Here, we describe a phage tailspike protein, named K2-2, that specifically depolymerizes the K2 capsular polysaccharide (CPS) of K. pneumoniae into tetrasaccharide repeating units. During the initial stage of infection, the tailspike proteins (TSPs) of bacteriophage recognize specific polysaccharides on the surface of the host cell and attach to them for adsorption. TSPs, also known as polysaccharide depolymerases, have the function of binding and digesting CPS. TSPs typically consist of three domains: an N-terminal particle-binding domain that connects to the tail structure or baseplate of the phage, a receptor-binding domain that extends from the homotrimeric structure and is responsible for host recognition and catalytic activity, and a C-terminal domain that plays a vital role in trimer formation, receptor binding, and intra-molecular chaperone functions.

Before the trimeric wild-type structures were determined using the N-terminally His-tagged protein, the first crystals of K2-2 were, indeed, obtained by using a C-terminally His-tagged protein (termed K2-2C-His). The structure was solved at 2.17 Å resolution by the MAD phasing method under the space group of P63. Unexpectedly, the solved structure revealed four protomers of the enzyme in an asymmetric unit, which formed a tetramer without the presence of a trimer. Specifically, two subunits are assembled into a dimer of a parallel left-handed helix, and two such dimers combine to form a right-handed superhelix. The two dimers superimpose well with each other, and also with any two adjacent subunits in the trimeric wild-type structure, presumably sharing a common interface. Regardless of the different overall organization, individual subunit in the tetrameric structure of K2-2C-His exhibited a conformation nearly identical to that in the trimeric form. The intersubunit carbohydrate-binding groove could be overlaid well with that of the trimeric structure (Cα rmsd = 0.29 Å), including the residues involved in binding the sugar (Fig. 5B through C). Notably, as determined by top agar assay, this tetrameric form of K2-2C-His possessed a significant capsule degradation activity towards the K2 K. pneumoniae. Conceivably, although the electron density corresponding to the C-terminal His-tag was not visible in all subunits, the protruding His-tag might give rise to steric hindrance that interfered with the assembly of the enzyme into a trimer. Finally, the structural and functional characterization of the tetrameric form of K2-2 here demonstrates, for the first time in the field of TPSs, that a functional intersubunit catalytic center could be formed without the need for trimerization.

>MALVDLVRAGGYSVEYPQFSSMAKLKAFPHSEDGQLVRLLSWHEGVGLGGGLFKVSTSSTATGNDGTVVVASNGVRLLRVVNGPIWADMFGALPNSDIDSMPAVAAAYAYAASVNTDLYIGVATYKFKGSTPINVDPSRAGIIGYQGKVRIDCSEFTGSIVFSINSSYSYTPAAYYNNLSPALQGLYVFGAKTSGVDGLLVGRETVGSDKSYNGQTEVRECTFDKFDRNIRMGHNSWRFVFYKVNSLNALSPNGILYVPAGLDDSGEILSFYHCQFFDGAGSNIRLSCSSYTMVFNTCSFLNITFFVDSASSATVTCNGCNFENPGSASTRRYVDISAGHTNVFNIIGGSIVTNSNPGQTQALLYVSTDNLLNLVGVTAPYGGHYQQEQELGYHAFIGGAGTVTTSGVMLQLRNGAGTCPLHSSLSTFSNWNFGYGNLNAWTVDKGTGTSSVVEYLANAGPKGTEGAMRVAPVSVGTNVSQVQAVTNPGMFSMSCMVNIATTPGNAGQVSIGFLDAAGNSLPGGVSANLGTTTGWQVIGKNTLRGKVPIGAKQVRVNIQTVAGADVKYAYLLCNVVKPLEHHHHHH[4x]>MASMTGGQQMGRDQAGITGTWYNQLGSTFIVTAGADGALTGTYESAVGNAESRYVLTGRYDSAPATDGSGTALGWTVAWKNNYRNAHSATTWSGQYVGGAEARINTQWLLTSGTTEANAWASTLVGHDTFTKVKPSAASIDAAKKAGVNNGNPLDAVQQGSGGGNGGGNGGGNGGGNIDGRGGGNASMTGGQQMGRDQAGITGTWYAQLGDTFIVTAGADGALTGTYVTARGNAESRYVLTGRYDSAPATDGSGTALGWTVAWKNNYRNAHSATTWSGQYVGGAEARINTQWLLTR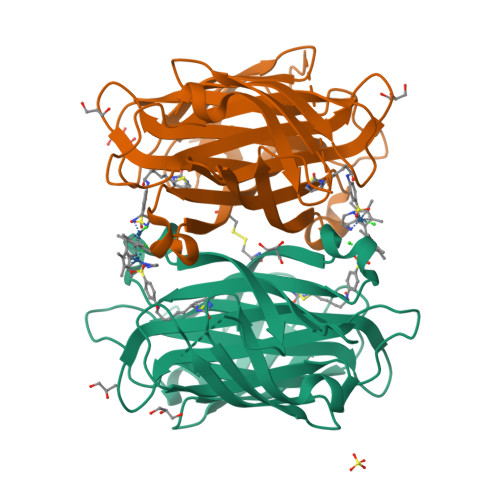GTTEANAWKSTLVGCATFTKVKPSAASIDAAKKAGVNNGNPLDAVQQ[2x]> SGETSVPPGSALVGPSCVMDDFRDPQRWKECAKQGKMPCYFDLIEENVYLTERKKNKSHRDIKRMQCECTPLSKDERAQGEIACGEDCLNR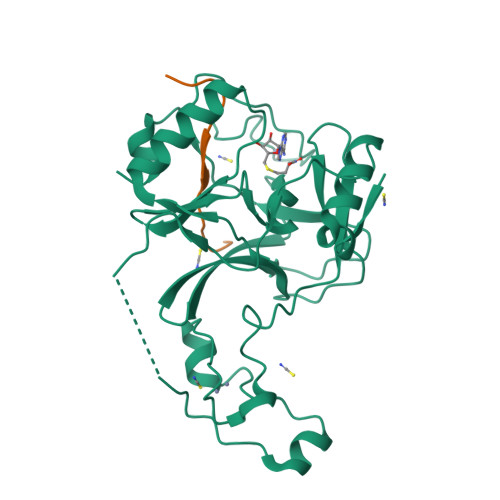LLMIECSSRCPNGDYCSNRRFQRKQHADVEVILTEKKGWGLRAAKDLPSNTFVLEYCGEVLDHKEFKARVKEYARNKNIHYYFMALKNDEIIDATQKGNCSRFMNHSCEPNCETQKWTVNGQLRVGFFTTKLVPSGSELTFDYQFQRYGKEAQKCFCGSANCRGYLGGENRVSIRAAGGKMKKERSRK;> APSTGGVMKPHRYR(4-{[(1S,2S)-2-(carboxymethyl)cyclopentyl]methyl}phenyl)acetic 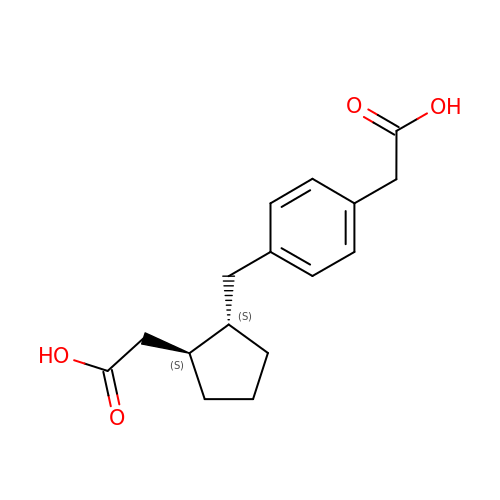acid | C16 H20 O4 | QKXFMUHRVZWRPO-KBPBESRZSA-N> K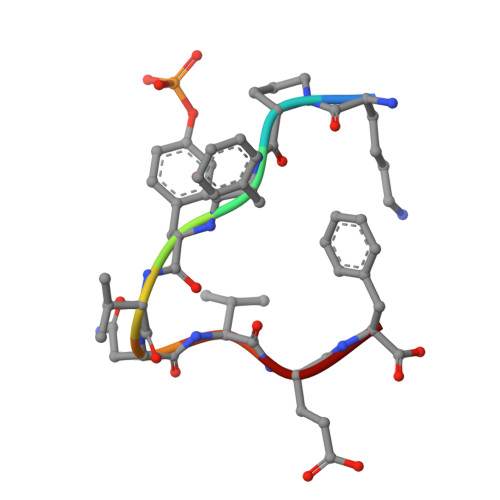PFYVNVEF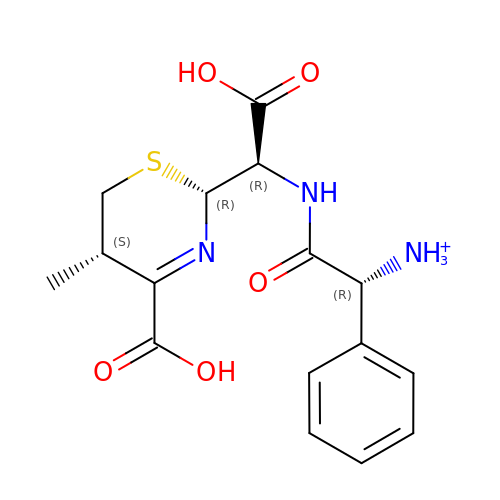(1R)-2-({(R)-carboxy[(2R,5S)-4-carboxy-5-methyl-5,6-dihydro-2H-1,3-thiazin-2-yl]methyl}amino)-2-oxo-1-phenylethanaminium | C16 H20 N3 O5 S | IEICSSILTYFRBD-QLXFMQRKSA-O>MGSGSSSYRPKAIYLDIDGRIQKVIFSKYCNSSDIMDL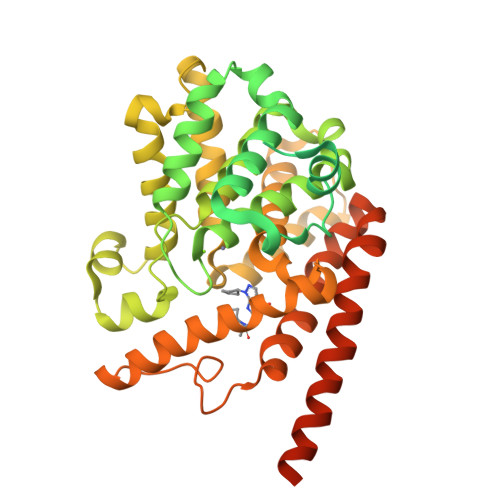FCIATGLPRNTTISLLTTDDAMVSIDPTMPANSERTPYKVRPVAIKQLSEREELIQSVLAQVAEQFSRAFKINELKAEVANHLAVLEKRVELEGLKVVEIEKCKSDIKKMREELAARSSRTNCPCKYSFLDNHKKLTPRRDVPTYPKYLLSPETIEALRKPTFDVWLWEPNEMLSCLEHMYHDLGLVRDFSINPVTLRRWLFCVHDNYRNNPFHNFRHCFCVAQMMYSMVWLCSLQEKFSQTDILILMTAAICHDLDHPGYNNTYQINARTELAVRYNDISPLENHHCAVAFQILAEPECNIFSNIPPDGFKQIRQGMITLILATDMARHAEIMDSFKEKMENFDYSNEEHMTLLKMILIKCCDISNEVRPMEVAEPWVDCLLEEYFMQSDREKSEGLPVAPFMDRDKVTKATAQIGFIKFVLIPMFETVTKLFPMVEEIMLQPLWESRDRYEELKRIDDAMKELQKKTDSLTSGATEKSRERSRDVKNSEGDCA[2x]> GPMGSKQMGSMHPVQVIAVTGGKGGVGKT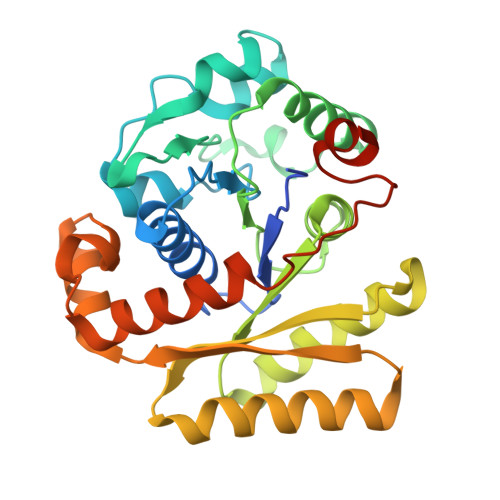NVSVNLALALADLGRRVMLLDAALGLANVDVLLGLTPKRTLADVIEGRCELRDVLLLGPGGVRIVPAASGTQSMVHLSPMQHAGLIQAFSDISDNLDVLVVDTAAGIGDSVVSFVRAAQEVLLVVCDEPTSITDAYALIKLLNRDHGMTRFRVLANMAHSPQEGRNLFAKLTKVTDRFLDVALQYVGVIPYDESVRKAVQKQRAVYEAFPRSKASLAFKAVAQKVDSWPLPANPRGHLEFFVERLVQHPATGSAV>[2x]MAHHHHHHMNCLFCKIAQGEIPATVVFEDKNILAFRD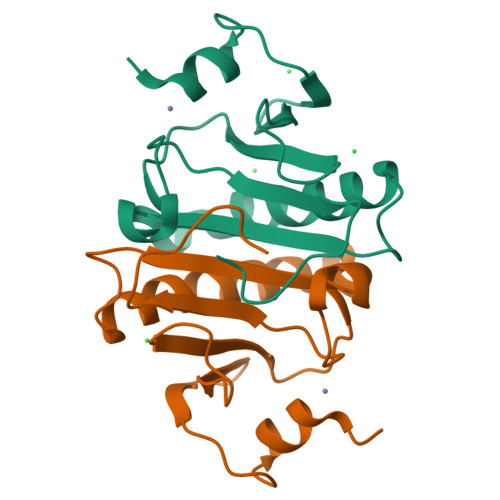IRPQAPTHLLIIPKKHIATINDVNDDDSELLANILIRAKKLAQAEGLSEMGYRLVFNVNSGGGQEVYHIHLHLLGGRQMTWPPG>GSHMGPSLDFALSLLRRNVRQVQTDQGHFTMLGVRDRLAVLPRHSQPGKTIWIEHKLVNVLDAVELVDEQGVNLDLTLITLDTNEKFRDITKFIPENISTASDATLVINTEHMPSMFVPVGDVVQYGFLNLSGKPTHRTMMYNFPTKAGQCGGVVTSVGKIIGIHIGGNGRQGFCAGLK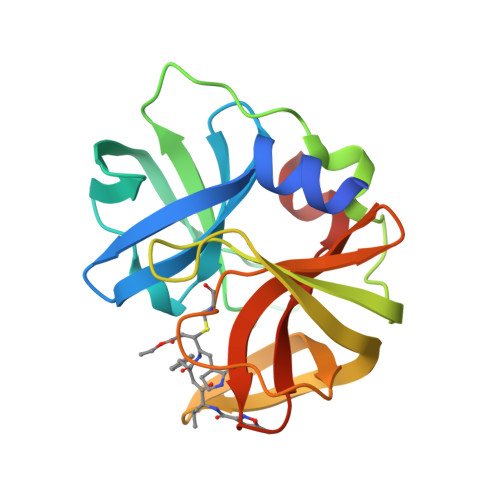RSYFASEQ[4x]> SEISRQEFQRRRQALVEQMQPGSAALIFAAPEVTRSADSEYPYRQNSDFWYFTGFNEPEAVLVLIK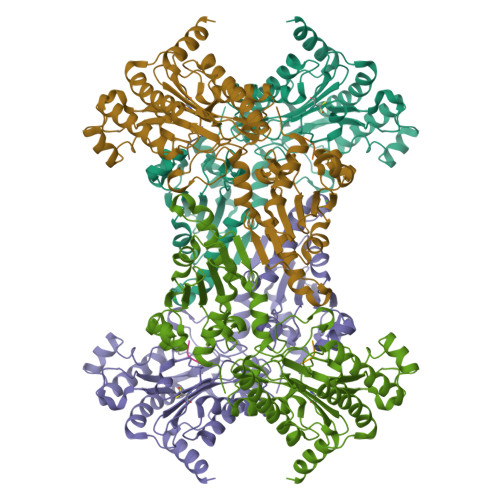SDDTHNHSVLFNRVRDLTAEIWFGRRLGQDAAPEKLGVDRALAFSEINQQLYQLLNGLDVVYHAQGEYAYADVIVNSALEKLRKGSRQNLTAPATMIDWRPVVHEMRLFKSPEEIAVLRRAGEITAMAHTRAMEKCRPGMFEYHLEGEIHHEFNRHGARYPSYNTIVGSGENGCILHYTENECEMRDGDLVLIDAGCEYKGYAGDITRTFPVNGKFTQAQREIYDIVLESLETSLRLYRPGTSILEVTGEVVRIMVSGLVKLGILKGDVDELIAQNAHRPFFMHGLSHWLGLDVHDVGVYGQDRSRILEPGMVLTVAPGLYIAPDAEVPEQYRGIGIRIEDDIVITETGNENLTASVVKKPEEIEALMVAARKQ;> VPL> MKKILIICMLFTLSFGIERPKFEDFLAGYERNKASMLNYEGMPAFALSENLLAVLKQPNTKLNKYVKYDPFLNLYLVRTDFSLIPTPMGDEEKLTRNDWVGIWDPNKPYIGHIKYLAQNIDEKDQLDFNSKIGLLGTPCCEMMGIALNNSSFIGNRY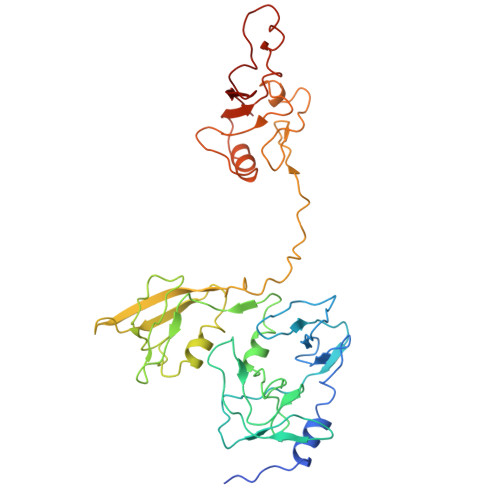LKHFMKYNDVYWGDIGVDFVVRENKIYVNNVRKNPQFLINDQVISVDGLPANDLRKLNEKILFADRGSTLYFQVLRDNMDLNISTEVFAKDLSKFNLPDSKPKPKITNFTSNLGLTVNTSLVVTKIDPKSKASNAGFMVGDKILRVNNIILNNFKELQNILSAGNDFSILIERKSTKLPLSNFNNELGGNANSGGDGKFQFFIRLTK> PISPIETVPVKLKPGMDGPKVKQWPLTEEKIKALVEICTEMEKEGKISKIGPENPYNTPVFAIKKKDGTKWRKLVDFRELNKKTQDFWEVQLGIPHPAGLKKKKSVTVLDVGDAYFSVPLDEDFRKYTAFTIPSINNETPGIRYQYNVLPQGWKGSPAIFQSSMTKILEPFRKQNPDIVIYQYMDDLYVGSDLEIGQHRTKIEELRQHLLRWGLTTPDKKHQKEPPFLWMGYELHPDKWTVQPIVLPEKDSWTVNDIQKLVGKLNWASQIYPGIKVRQLCKLLRGTKALTEVIPLTEEAELELAENREILKEPVHGVYYDPSKDLIAEIQKQGQGQWTYQIYQEPFKNLKTGKYARMRGAHTNDVKQL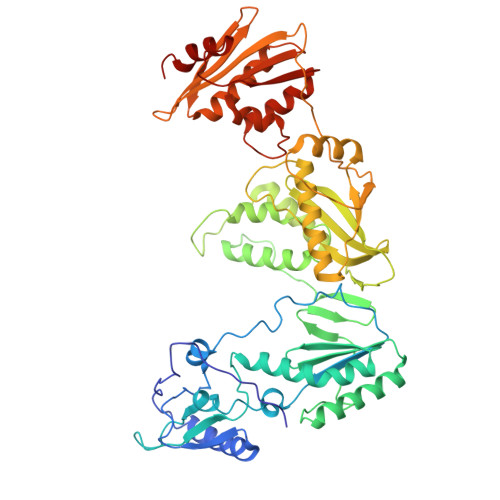TEAVQKITTESIVIWGKTPKFKLPIQKETWETWWTEYWQATWVPEWEFVNTPPLVKLWYQLEKEPIVGAETFYVDGAASRETKLGKAGYVTNKGRQKVVTLTDTTNQKTELQAIHLALQDSGLEVNIVTDSQYALGIIQAQPDQSESELVNQIIEQLIKKEKVYLAWVPAHKGIGGNEQVDKLVSAGIRKIL>SMDSLNFGKALEALKEGK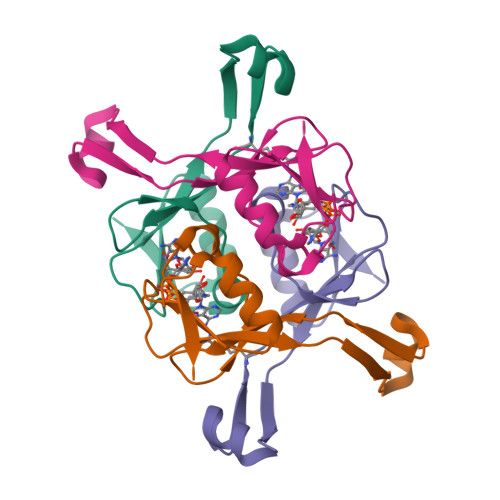KVSREGWNGKGMFAYYVPGGVYKSQTDVIKNTFGEEVKYRPYLALKTVDNDIATWTPSVSDILAEDWNIVE[2x]>[3x]AAY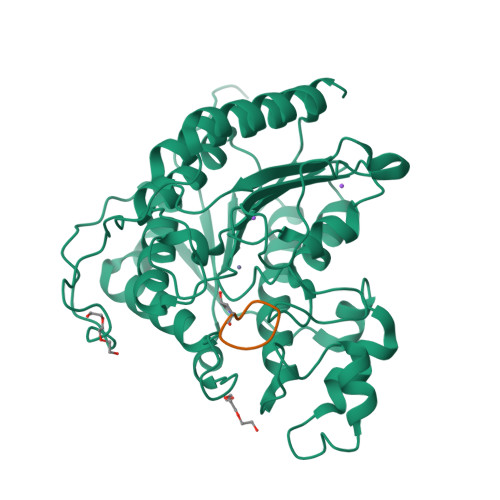SQGGGKKKVCYYYDGDIGNYYYGQGHPMKPHRIRMTHNLLLNYGLYRKMEIYRPHKATAEEMTKYHSDEYIKFLRSIRPDNMSEYSKQMQRFNVGEDCPVFDGLFEFCQLSTGGSVAGAVKLNRQQTDMAVNWAGGLHHAKKSEASGFCYVNDIVLAILELLKYHQRVLYIDIDIHHGDGVEEAFYTTDRVMTVSFHKYGEYFPGTGDLRDIGAGKGKYYAVNFPMRDGIDDESYGQIFKPIISKVMEMYQPSAVVLQCGADSLSGDRLGCFNLTVKGHAKCVEVVKTFNLPLLMLGGGGYTIRNVARCWTYETAVALDCEIPNELPYNDYFEYFGPDFKLHISPSNMTNQNTPEYMEKIKQRLFENLRMLPHAPGVQMQAI;>XNPKQKWG[3x]[1-(3-CHLORO-2-FORMYL-PHENYLCARBAMOYL)-2-METHYL-PROPYL]-CARBAMIC 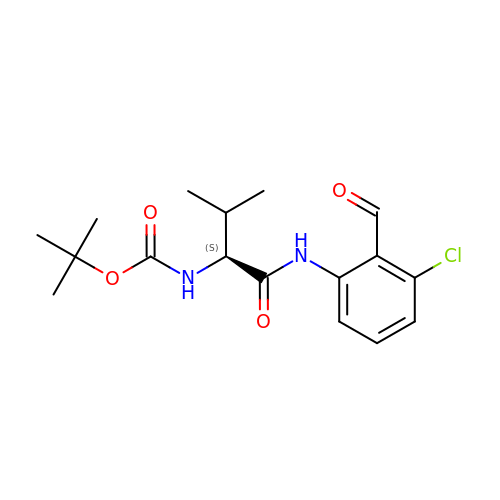ACID TERT-BUTYL ESTER | C17 H23 Cl N2 O4 | GBHYPZDGTWSQFR-AWEZNQCLSA-N> MEDNLINVLSINERCFLLKQSGNEKYDIKNLQAWKERKSVLKQDDLDYLIKYKYESLDNFGLGITPIENFPDKEVAIQYIKDQSWYIFFESILDSYNDSEEQLLEVDASYPFRYFLQYARLFLLDLNSELNICTKEFIINLLEILTQE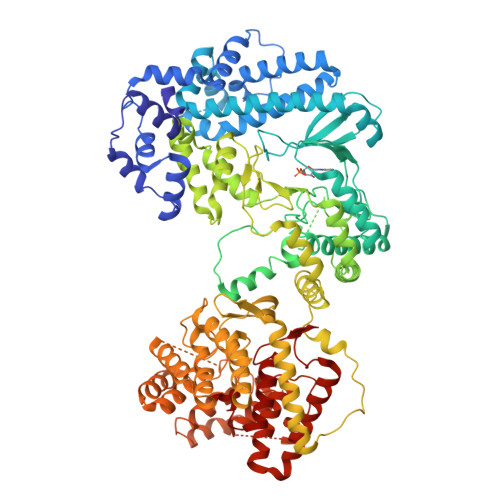LIHLTSKTLVLDLHTFKKNEPLKGNDSSKRFIYYLKKRFNSKKDIIAFYTCYPELMRITVVRMRYFLDNTKQMLIRVTEDLPSIQNCFNIQSSELNSISESQGDSHSRGKTVSTLTFSDGKKIVYKPKINSENKLRDFFEFLNKELEADIYIVKKVTRNTYFYEEYIDNIEINNIEEVKKYYERYGKLIGIAFLFNVTDLHYENIIAHGEYPVIIDNETFFQQNIPIEFGNSATVDAKYKYLDSIMVTGLVPYLAMKDKSDSKDEGVNLSALNFKEQSVPFKILKIKNTFTDEMRFEYQTHIMDTAKNTPIMNNEKISFISYEKYIVTGMKSILMKAKDSKKKILAYINNNLQNLIVRNVIRPTQRYADMLEFSYHPNCFSNAIEREKVLHNMWAYPYKNKKVVHYEFSDLIDGDIPIFYNNISKTSLIASDGCLVEDFYQESALNRCLNKINDLCDEDISIQTVWLEIALNIYNPYKYINDLKNQNSNKYIYTGLELNGKIIQACQKIEKKIFKRAIFNKKTNTVNWIDIKLDQDWNVGILNNNMYDGLPGIFIFYVALKYITKNHKYDYVIECIKNSIYTIPSEDILSAFFGKGSLIYPLLVDYRLNNDINSLNVAVEIADMLIEKKPINNGELKNDWIHGHNSIIKVLLLLSEITEDEKYRKFSLEIFEKLSEEPYFNFRGFGHGIYSYVHLLSKFNRIDKANSLLHKIKESYFEEEPKNNSWCKGTVGELLATIELYDDNISNIDINKTIEYKNKDCLCHGNAGTLEGLIQLAKKDPETYQYKKNKLISYMLKYFEKNNTLKVAGSEYLESLGFFVGISGVGYELLRNLDSEIPNALLFEL> AWATEQKTEEIPPPDLYKDTPAWYQAVYKDNVGLSEGSGPFTKYFKAQMLDMYWQPNRHYEPMENLDHSIFIEQERRDLCVICHEEATPGIVADWRSSGHKHPKSTPYLSSKTAQIEKNVGRVLDEVHCFDCHADTEKNQIRMPTGEVCGGCHRQQFDEFLREREVGRPNHLQSWEANTIVPWYAEAARRGYLYGQHGCDMCHSGAEKCDVCHTRHKFSAVEGRQPEACMTCHMGPDHPDAESYGESKHGKIYEKEEEHYDFTKPLVEVRPGEDYRTPTCQYCHMYEKHGRFIHNPVMKGIWRMGTVPPSNLEYTSSLKDYPYGIKIIADKIDIYSEENVAKRSYWLEVCAKCHSDRFADTYLKSLDQFMFQAHTLADQAQKIVEDLIADGLLYPDAAN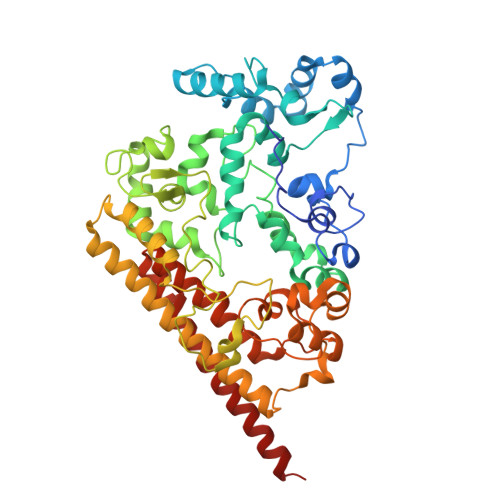RDPYPLSDGIVKELSADFLGEPVYNAFKTLQGKFPVVGPILGVYGMFLQMQDNPSDIENMYNRLWFWYKLQGYKGTAHAQQDVSWWWGQAPMMMEMTRIQAEAARLRRLAGIEKTISK>GGTGPIFIKEVSNADISMGDVATLSVTVIGIPKPKIQWFFNGVLLTPSADYKFVFDGDDHSLIILFTKLEDEGEYTSMASNDYGKTICSAYLKINSKGEG[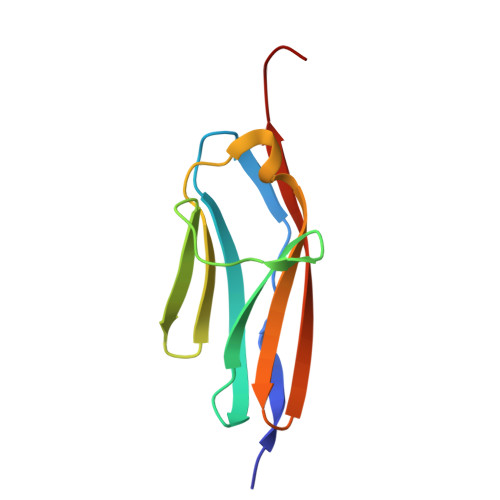6x]>[3x]MIKQRTLKNIIRATGVGLHSGEKVYLTLKPAPVD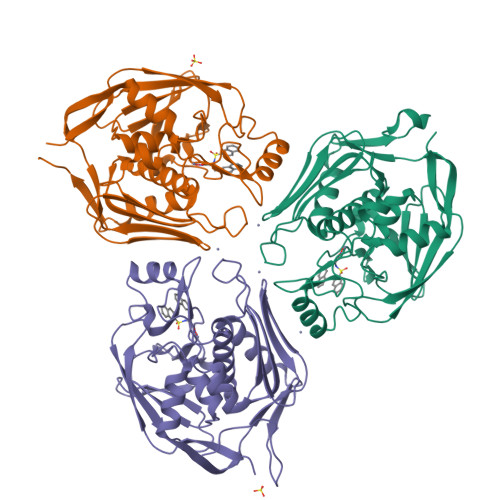TGIVFSRTDLDPVVEIPARAENVGETTMSTTLVKGDVKVDTVEHLLSAMAGLGIDNAYVELSASEVPIMDGSAGPFVFLIQSAGLQEQEAAKKFIRIKREVSVEEGDKRAVFVPFDGFKVSFEIDFDHPVFRGRTQQASVDFSSTSFVKEVSRARTFGFMRDIEYLRSQNLALGGSVENAIVVDENRVLNEDGLRYEDEFVKHKILDAIGDLYLLGNSLIGEFRGFKSGHALNNQLLRTLIADKDAWEVVTFEDARTAPISYMRP>ETGGCTNVDSPNFNFQANMDDDSCDAKVTNFTFGGVYQECTELSGDVLCQNLEQKNLLTGDFSCPPGYSPVHLLSQTHEEGYSRLECKK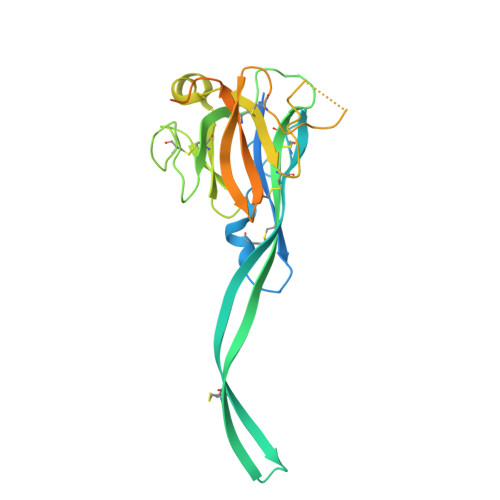KCTLKIFCKTVCEDVFRVAKAEFRAYWCVAAGQVPDNSGLLFGGVFTDKTINPMTNAQSCPAGYIPLNLFESLKVCVSLDYELGFKFSVPFGGFFSCIMGNPLVNSDTAKDVRAPSLKKCPGGFSQHLAVISDGCQVSYCVKAGIFTGGSLLPVRLPPYTKPPLMSQVATNTVIVTNSETARSWIKDPQTNQWKLGEGTKHHHHHH[8x]> MKIAGIDEAGRGPVIGPMVIAAVVVDENSLPKLEELKVRDSKKLTPKRREKLFNEILGVLDDYVILELPPDVIGSREGTLNEFEVENFAKALNSLKVKPDVIYADAADVDEERFARELGERLNFEAEVVAKHKADDIFPVVSAASILAKVTRDRAVEKLKEEYGEIGSGYPSDPRTRAFLENYYREHGEFPPIVRKGWKTTQDM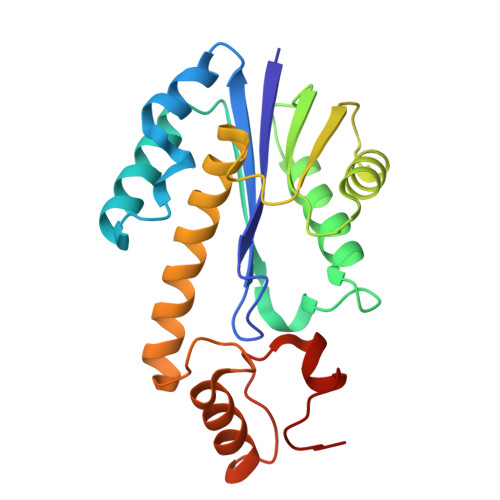INKST>[4x]LDGDQMISHRELWAKIANSINDINEYLKVYEHAVSSYTQMYQDFSAVLSSLAG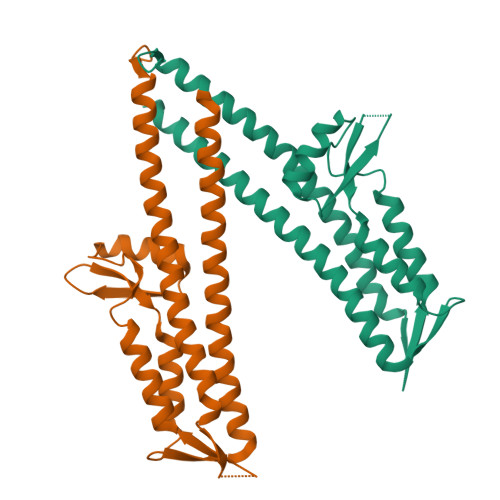WISPGGNDGNSVKLQVNSLKKALEELKEKYKDKPLYPANNTVSQEQANKWLTELGGTIGKVSQKNGGYVVSINMTPIDNMLKSLDNLGGNGEVVLDNAKYQAWNAGFSAEDETMKNNLQTLVQKYSNANSIFDNLVKVLSSTISS>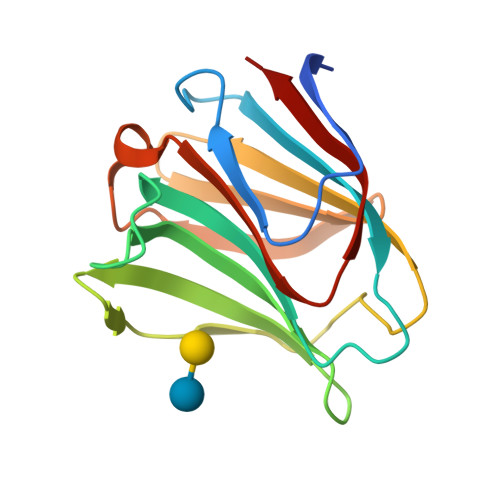MMLSLNNLQNIIYNPVIPFVGTIPDQLDPGTLIVIRGHVPSDADRFQVDLQNGSSVKPRADVAFHFNPRFKRAGCIVCNTLINEKWGREEITYDTPFKREKSFEIVIMVLKDKFQVAVNGKHTLLYGHRIGPEKIDTLGIYGKVNIHSIGFSFS[4x]>GHMKDLKGTKTAENLKQGFIGESMANRRYL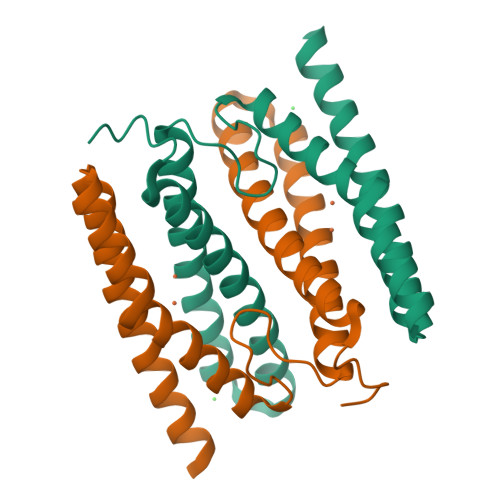YFAKRADEEGYPEIAGLLRSIAEGETAHAFGHLDFIRQGGLTDPATDKPIGTLEQMIESAIAGETYEWTQMYPGFAKVAREEGFPEVAEWFETLARAEKSHAEKFQNVLKQLKGGT[2x]>SNAMTKKKVYIVSHSHWDREWYLPYEEHHMRLIELVDNVLDLIENDPEFNSFHLDGQTIILDDYLQVRPEKKEAVKKAVQAGKLKIGPFYILQDDFLISSESNVRNMLIGHLESQKWGAPVQLGYFPDTFGNMGQTPQMMQLANLPAAAFGRGVKPIGFDNQVLESDYSSQYSEMWWEGPDQTKIFGLLFANWYSNGNEIPSEKEAAIAFWKQKLADVERYASTNHLLMMNGVDHQPVQRDITKAIALANELFPEYEFIHSNFDDYLKAVQEELPEDLGTVTGELTSQETDGWYTLANTSSARVYLKQWNTKVQRQLENIAEPLAAMAYEVTGDYPHDQFDYAWKTLLQNHPHDSICGCSVDEVHRGMMTRFENANDVGHFLADEATRQLTEAIDTSVFPEKAHPFVLFNTSGYQKTEVVTVEVEIERLPFYTGKPEDLYHELKQKATPDYQVIDPTGKAVASRIVKEDVRFGYDLPKDAFRQPYMAKYLTVELSVKEMAPFSWDSFALIQGETKAFEGSLLAQPATNEMENEFIQVKIENNGSLTIADKKTGETFSKLLTFEDTGDIGNEYIFFKPTEDQGITTENVTAEITNKENSPVKASYQIKQTVMLPVAADERLEEEQKAVREFRERLAQRSTTLRPFEITTMVTMIKESNQLFFETTINNQIKDHRLRVLFPTGMVTETHEADSIYEVVTRPNQVSDTWENPTNPQHQQAFVNVHDQNKGVTIFNEGLNEYEVLADGTIAVTLIRCVGELGDWGYFATPEAQCQGEYTFKYGLSLHGKPEERFATYQQAYSAQIPFTAATTARHEGKLAPNHVYLTHAEGPIGWTAVKRQEQTNHLVVRGFNLTAQNIPCELHKETQP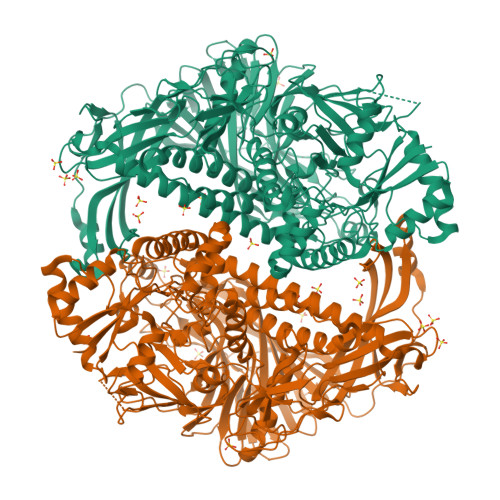ATCLTNVLEEPLTPAIEVDAPLRPFEIRTWRFEK[2x]>MKKILSIFIVVFLFAVGCGQQKEEKKE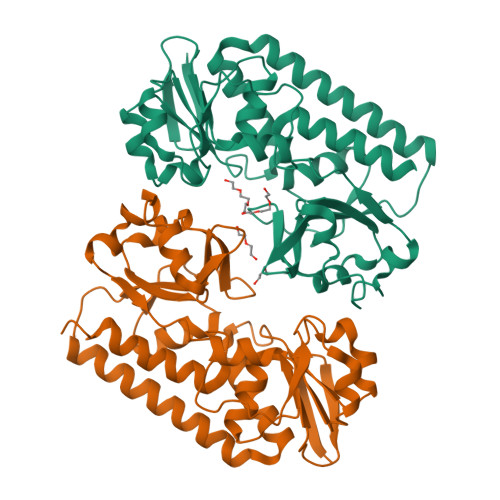TKADNKNQAITIKHAEGETKLDKPAKKVVVLEWVYSEDLLALGVQPVGMADIKNYNKWVNTKTKPSKDVVDVGTRQQPNLEEISRLKPDLIITASFRGKAIKNELEQIAPTVMFDPSTSNNDHFAEMTETFKQIAKAVGKEEEGKKVLADMDKAFADAKAKIEKADLKDKNIAMAQAFTAKNVPTFRILTDNSLALQVTKKLGLTNTFEAGKSEPDGFKQTTVESLQSVQDSNFIYIVADEDNIFDTQLKGNPAWEELKFKKENKMYKLKGDTWIFGGPESATSLATQVADVMTAKK[2x]>GSHMDEILARAGIFQGVEPSAIAALTKQLQPVDFPRGHTVFAEGEPGDRLYIIISGKVKIGRRAPDGRENLLTIMGPSDMFGELSIFDPGPRTSSATTITEVRAVSMDRDALRSWIADRPEISEQLLRVLARRLRRTNNNLADLIFTDVPGRVAKQLLQLAQRFGTQEGGALRVTHDLTQEEIAQLVGASRETVNKA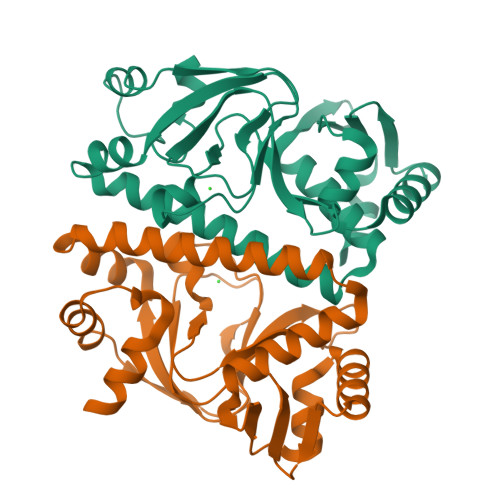LADFAHRGWIRLEGKSVLISDSERLARRAR[2x]>[2x]MPKALIVYGSTTGNTEGVAEAIAKTLNSEGMETTVVNVADVTAPGLAEGYDVVLLGCSTWGDDEIELQEDFVPLYEDLDRAGLKDKKVGVFGCGDSSYTYFCGAVD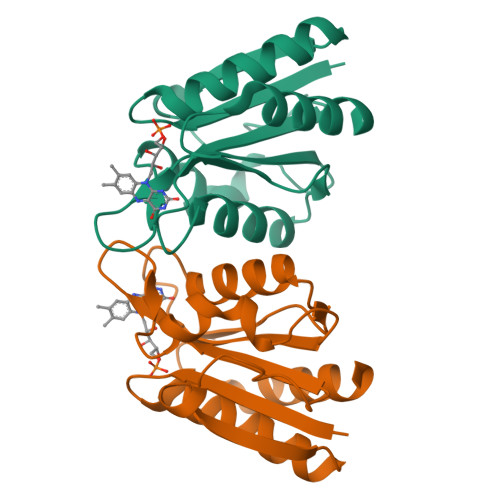VIEKKAEELGATLVASSLKIDGEPDSAEVLDWAREVLARV>[2x]TDEITSFSIPKFRPDQPNLIFQGGGYTTKEKLTLTKAVKNTVGRALYSLPIHIWDSETGNVAD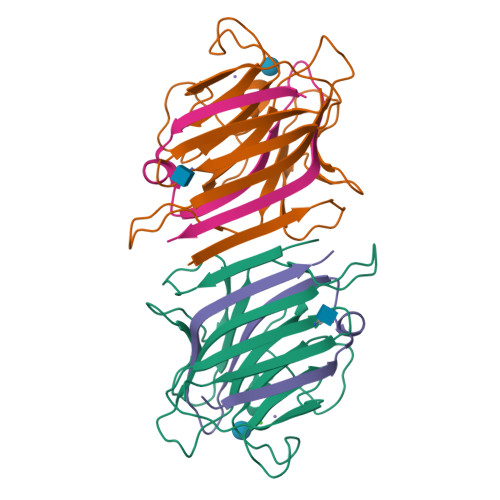FTTTFIFVIDAPNGYNVADGFTFFIAPVDTKPQTGGGYLGVFNGKDYDKTAQTVAVEFDTFYNAAWDPSNGKRHIGIDVNTIKSISTKSWNLQNGEEAHVAISFNATTNVLSVTLLYPN;>LTGYTLSEVVPLKDVVPEWVRIGFSATTGAEYATHEVLSWTFLSELTGPSN[2x]> MDHAIYTAMGAASQTLNQQAVTASNLANASTPGFRAQLNALRAVPVDGLSLATRTLVTASTPGADMTPGQLDYTSRPLDVALQQDGWLVVQAADGAEGYTRNGNIQVGPTGQLTIQGHPVIGEGGPITVPEGSEITIAADGTISALNPGDPPNTVAPVGRLKLVKAEGNEVQRSDDGLFRLTAEAQAERGAVLAADPSIRIMSGVLEGSNVK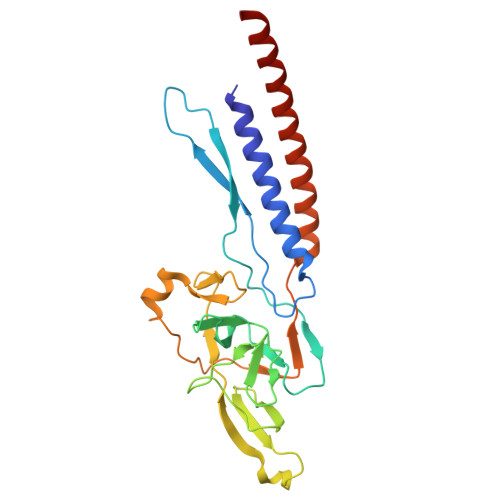PVEAMTDMIANARRFEMQMKVITSVDENEGRANQLLSMS BULGECIN A 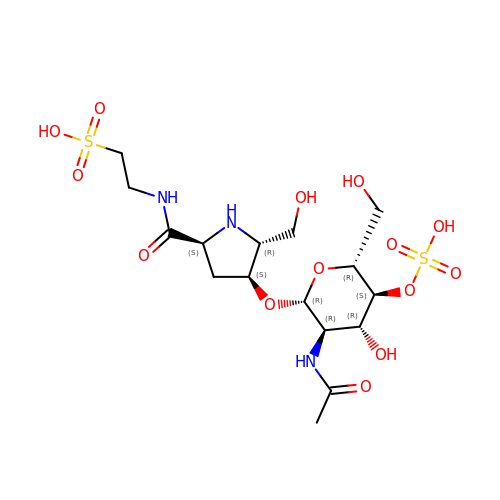| C16 H29 N3 O14 S2 | RPNZWZDLNYCCIG-HMMVDTEZSA-N> MSPATVLDSILEGVRADVAAREASVSLSEIKAAAAAAPPPLDVMAALREPGIGVIAEVKRASPSAGALATIADPAKLAQAYQD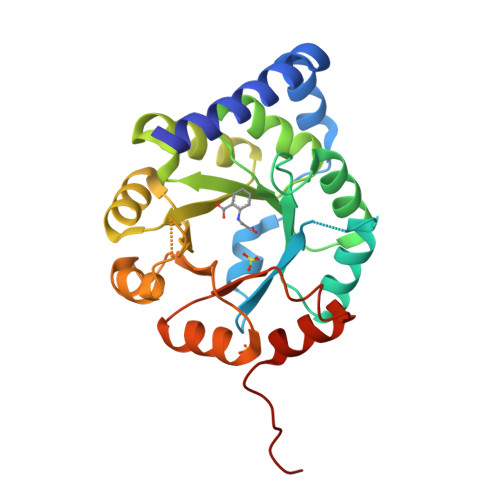GGARIVSVVTEQRRFQGSLDDLDAVRASVSIPVLRKDFVVQPYQIHEARAHGADMLLLIVAALEQSVLVSMLDRTESLGMTALVEVHTEQEADRALKAGAKVIGVNARDLMTLDVDRDCFARIAPGLPSSVIRIAESGVRGTADLLAYAGAGADAVLVGEGLVTSGDPRAAVADLVTAGTHPSCPKPAR>ALYEDPPDQKTSPSGKPATLKICSWNVDGLRAWIKKKGLDWVKEEAPDILCLQETKCSENKLPAELQELPGLSHQYWSAPSDKEGYSGVGLLSRQAPLKVSYGIGDEEHDQEGRVIVAEFDSFVLVTAYVPNAGRGLVRLEYR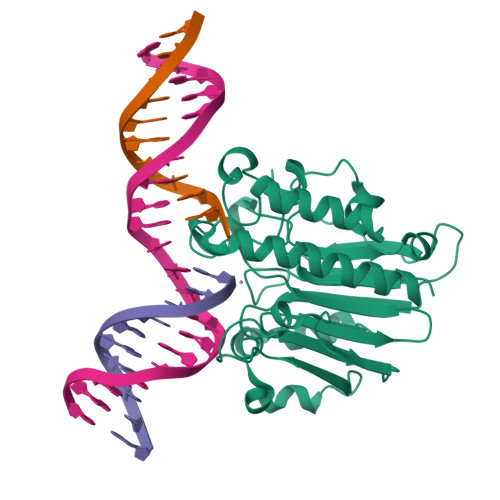QRWDEAFRKFLKGLASRKPLVLCGDLNVAHEEIDLRNPKGNKKNAGFTPQERQGFGELLQAVPLADSFRHLYPNTPYAYTFWTAMMNARSKNVGWRLDYFLLSHSLLPALCDSKIRSKALGSDHCPITLYLAL[2x]FURFURAL 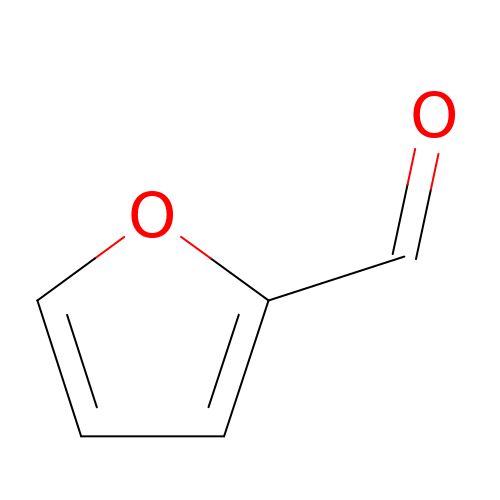| C5 H4 O2 | HYBBIBNJHNGZAN-UHFFFAOYSA-N> MSMIDEPLYPIAVLIDELKNDDIQLRLNSIRRLSTIARALGEERTRKELIPFLSENNDDDDEVLLAMAEELGVFIPYVGGVEYAHVLLPPLETLSTVEETCVREKAVESLCRVGSQMRESDLVDHFISLVKRLAAGEWFTARVSACGVFHIAYPSAPDMLKTELRSLYTQLCQDDMPMVRRAAATNLGKFAATVESAHLKTDVMSMFEDLTQDDQDSVRLLAVEGCAALGKLLEPQDCVQHILPVIVNFSQDKSWRVRYMVANQLYELCEAVGPEPTRTELVPAYVRLLRDNEAEVRIAAAGKVTKFCRILNPEIAIQHILPCVKELSSDSSQHVRSALASVIMGMAPVLGKDATIEHLLPIFLSLLKDEFPDVRLNIISKLDQVNQVIG;> SSVPGFEKLANLLKPKPGLKKLLKWADAKKPPETVFTRLRLDKTGTQLFDNTDFPVWAAYTRSVAQTDSEASAVMLKTLVSRYSDEVLSGMIAAAKKSSKTESIATKLETEQMRTWLAAKKTPDDMFLVFKLNKAGDDILSSPLLSAWTNYMKLSNKENPKAQTTLIATMT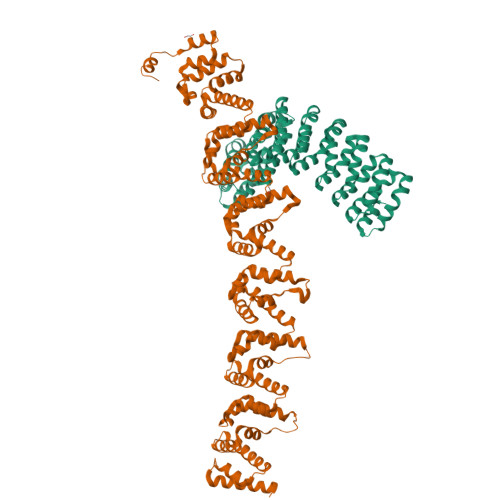KHYGDSGVSQILAAARKSPATQSTAKRLEAEQVQLWLKKGRTPDDTFTLLSLDRAGDDLLASPQFNTWMKYINYYNKENPDEKTTVLAKLMTHFDDEELTPILVVARKVPSTESTAAKLQAEQFKNWLSADKSPEEAFTLLQLDKAGDDLLTNPQLTNWLKYTENFNLNKEINEQVTAIQVFRAQYVDDSRIANMVIAAEKVPNTQAIAKRVEDELFKGWTVVLNKPDDVFINLKLETVGENVFESPLWSFYTKFLEKYNTANPGKEQTMISGLARGYNDVTLTNMLLKAKEAPSTKTLATKLEDELVQYWLADKKLPDKLFGYLELKESVDGILTNPVFNVWLKYLNAFNDKAPVKKALMIDTLKSAFGDVAVSNMLFAAKKDPGTAKVAATLQTALLSKWVLEKKTPGQVSAILKEGAGADVSAKLLATYSAKFKVRWG>[4x]GEELIKENMHMKLYMEGTVNNHHFKCTSEGEGKPYEGTQTMRIKVVEGGPLPFAFDILATSFMYGSRTFIN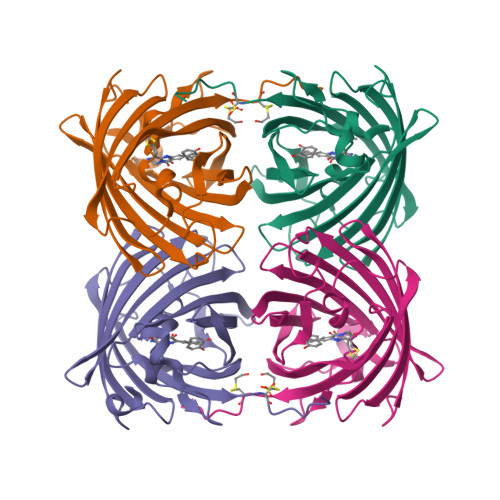HTQGIPDFFKQSFPEGFTWERVTTYEDGGVLTATQDTSLQDGCLIYNVKIRGVNFPSNGPVMQKKTLGWEANTEMLYPADGGLEGRTDMALKLVGGGHLICNFKTTYRSKKPAKNLKMPGVYYVDHRLERIKEADKETYVEQHEVAVARYCDLPSKLGHKLNGMDELYK> GPHMASMLEAKFEEASLFKRIIKGFKDCVQLVNFQCKEDGIIAQAVDDSRVLLVSLEIGVEAFQEYRCDHPVTLGMDLTSLSKILRCGNNTDTLTLIADNTPDSIILLFEDTKKDRIAEYSLKLMDIDADFLKIEELQYDSTLSLPSSEFSKIVRDLSQLSDSINIMITKETIKFVADGDIGSGSVIIKPFVDMEHPETSIKLEMDQPVDLTFGAKYLLDIIKGSSLSDRVGIRLSSEAPALFQFDLKSGFLQFFLAPKFNDEE

PCNA is a ring-shaped homotrimeric complex that encircles DNA to act as a sliding clamp, ensuring processivity of DNA polymerases. It also operates as a platform for recruitment of numerous other proteins involved in DNA replication, DNA damage repair, mismatch repair, and chromatin structure and assembly. PCNA levels on DNA are regulated by loading and unloading. After completion of each Okazaki fragment, the Elg1 RFC-like complex (Elg1-RLC), which comprises the Elg1 subunit associated with the Rfc2–5 subunits, functions to unload PCNA from the lagging strand.

We then constructed strains expressing each PCNA mutant as the only copy of the POL30 gene, expressed from its endogenous locus, and found two PCNA mutants PCNA-D17K and PCNA-D21K that accumulate on DNA even with Elg1 present. Retention-prone mutants PCNA-D17K and PCNA-D21K have point mutations on the DNA-interacting region of inner ring. Elg1 can physically interact with PCNA-D17K and actually shows enhanced interaction with PCNA-D21K, suggesting that accumulation of those PCNA mutants on DNA is not due to a loss of interaction with the Elg1-RLC unloader. These retention-prone mutants increase the mutation rate even in the presence of Elg1 (columns 3 and 5), suggesting that PCNA accumulation on DNA alone and/or the D17K and D21K mutations themselves can increase the mutation rate. The structures (at 2.80- and 2.85-Å resolution for PCNA-D21K and PCNA-D17K, respectively) reveal that the mutations alter the inner pore of the PCNA ring. In both cases, the PCNA pore becomes more electropositive due to the swap of a negative charge to a positive charge. For D17K, lysine 17 is positioned within the major groove of DNA, where the electrostatic interaction with DNA is also enhanced. The D17K mutation on the other hand disrupts a salt bridge network within the PCNA pore, resulting in partial unraveling of helix 1, and a conformational change of an adjacent loop (residues 20 through 25). Because this conformational change occurs on the primary interaction face of PCNA, the D17K variant could potentially perturb binding of PCNA partner proteins. To avoid this complication, we focused our further analyses primarily on the D21K variant.> SAASNPSIS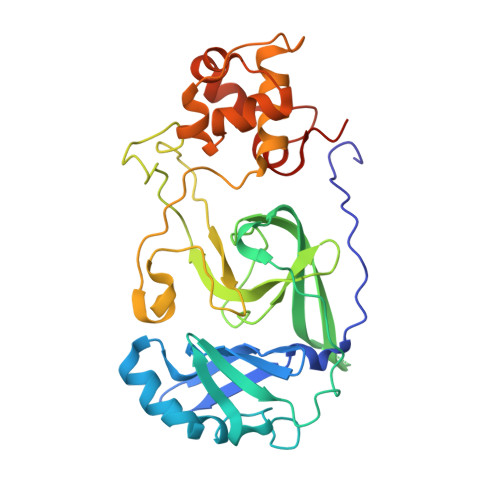HIVLEMPVAINPLIKYTTRTSVSSLRGAVVNGYIYIQRHLFGSKKQEFEACYNNGKGLLNCKNLERSKYDIDSAELIGTLIRIPLHDKHSIPHISIHPDPLSYNGPVTLYLSRYDTELNKDVLCVHTGFMSEGHHDIKTVFGDCGGMLFDPKGRLLGLHCAGSDDVVFMDTTTGKSNIWTSYKLQHPSEIMITLNNEINLPNPANYDFETTKVVYQHPLRNVCATLETLQHLTNKTNAKLPYDSRLLSDFNITAEQYNQYGYYIDYNNFVNNFNRYTTTTIGTKSFETCIKYGLMDNKKPDYYNQ> MFLGIFKDVIKLLNKKVVPVYFWFFLYCFLSTMDTNIFVSSCSFLKVEVFGKDENTTLVLLFYVFYSLFNFYLSRIKNKNNYLVRKHLYTTELLIELILFKYK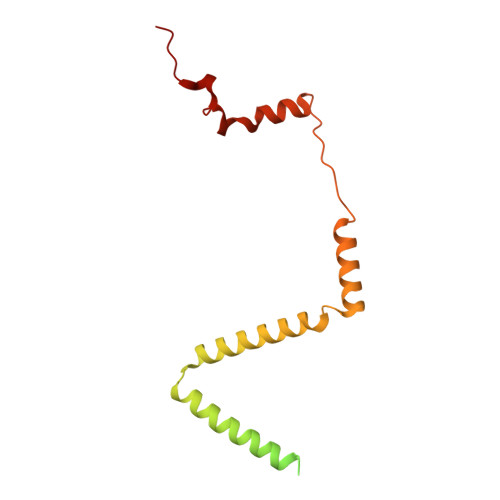LIILKFSSIKYILNFNVRKFILFNLFLINNYKAYKINTFFLYIYIYLNNLNIIWYPIFKAYSIFGYYKSTRLNFIDTKNENIKRIKY>[2x]MILDINDVLGKKIITTRLMSSITIHEENSIAALEVMSRFAADPHWLIYLPPTMSPCETSKKEGMLEHPIEAFEYFRTRGVGKVVCEQKHMGSRAVVIVCKDSQVAEKRFGVLDGTAGICYTRTGRHFFDDMQLEAELIDRVRKVLDKSGFWGDFNTDWVCLDCELMPWSAKAQKLLEEQYSAVGISGRVVLDEAVKLLKQASLNKTVSFDVSRQTSGKNADINELLQRFTERSEMMQKYVEAYRKYCWPVNSIDDLKLAPFHILATEGKVHSDKNHIWHMDTIAKYCTQDDSLIMATNHILVDVTDAESVDKGIKWWEDLTASGGEGMVVKPYDFIVKNGRELLQPAVKCRGREYLRIIYGPEYTMDENIERLRNRAVGKKRSLALREFSLGMEALERFVRNEPLYRVHECVFGVLALESEPVDPRL;>MILTITYTQPPATDLG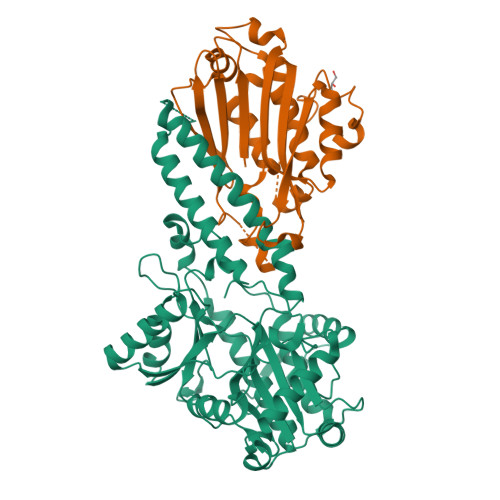YLLHKNPSRPQTFELNHGKAHIFYPEATSERCTVALLLDIDPIDLARGKKGSSGEGGLFDYVNDRPYVSSSFMSVAISRVFGTAMSGKCKEKPELAAIKLPLKAKIMMLPCKGGEEIIYRLFEPLGYKVDVEGYMLDEKFPEWGKSRYYTVSLEGEVRVRDLLNHIYVLIPVLDSEKHYWVGEDEIDKLFQHGEGWLVDHPEKELITGRYLIRK[2x]>[2x]SNADQTYCDRLVQDTPFLTGHGRLSEQQVDRIILQLNRYY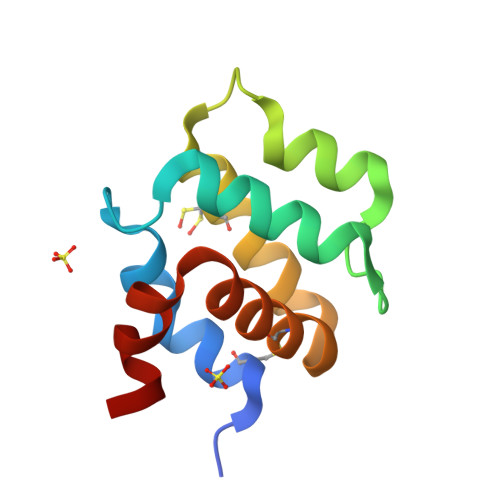PQILTNKEAEKFRNPKASLRVRLCDLLSHLQRSGERDCQEFYRALYIHAQPLHSRLPSRH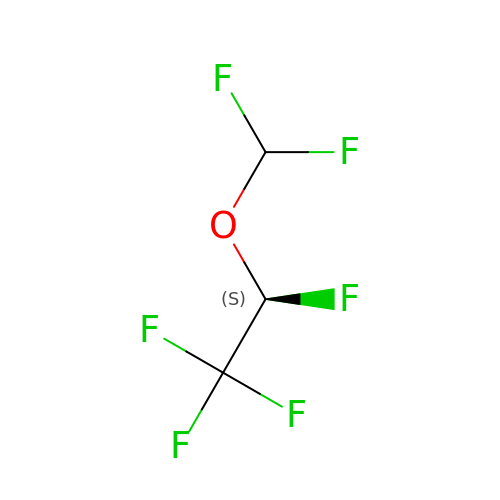(2S)-2-(difluoromethoxy)-1,1,1,2-tetrafluoroethane | C3 H2 F6 O | DPYMFVXJLLWWEU-PVQJCKRUSA-N>MGHHHHHHGSLVPRGSRAYSFKVVLLGEGCVGKTSLVLRYCENKFNDKHITTLQASFLTKKLNIGGKRVNLAIWDTAGQERFHALGPIYYRDSNGAILVYDITDEDSFQKVKNWVKELRKMLGNEICLCIVGNKIDLEKERHVSIQEAESYAESVGAKHYHTSAKQNKGI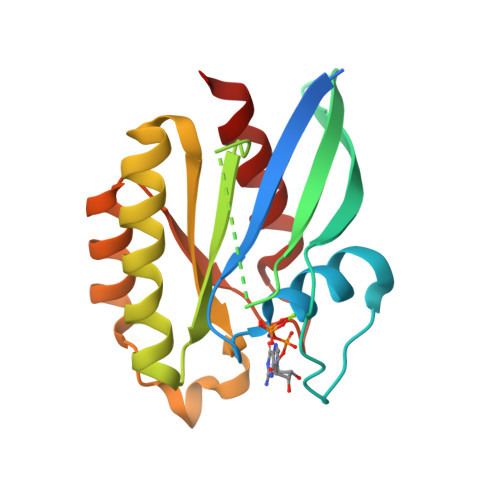EELFLDLCKRMIET[2x]> SVDDFISTETPIALNNLLCNVGPDGCRAFGTSAGAVIASPSTIDPDYYYMWTRDSALVFKNLIDRFTETYDAGLQRRIEQYITAQVTLQGLSNPSGSLADGSGLGEPKFELTLKPFTGNWGRPQRDGPALRAIALIGYSKWLINNNYQSTVSNVIWPIVRNDLNYVAQYWNQTGFDLWEEVNGSSFFTVANQHRALVEGATLAATLGQSGSAYSSVAPQVLCFLQRFWVSSGGYVDSNINTNEGRTGKDVNSVLTSIHTFDPNLGCDAGTFQPCSDKALSNLKVVVDSFRSIYG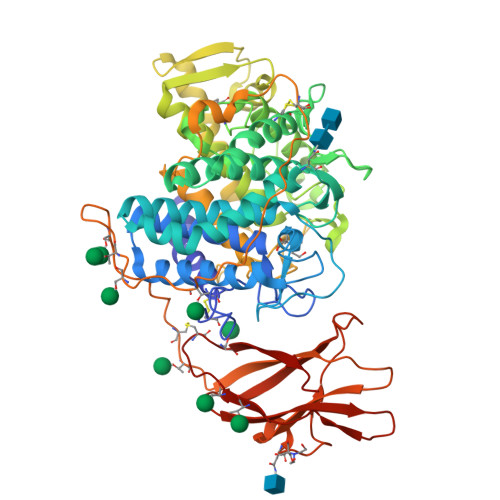VNKGIPAGAAVAIGRYAEDVYYNGNPWYLATFAAAEQLYDAIYVWKKTGSITVTATSLAFFQELVPGVTAGTYSSSSSTFTNIINAVSTYADGFLSEAAKYVPADGSLAEQFDRNSGTPLSALHLTWSYASFLTATARRAGIVPPSWANSSASTIPSTCSGASVVGSYSRPTATSFPPSQTPKPGVPSGTPYTPLPCATPTSVAVTFHELVSTQFGQTVKVAGNAAALGNWSTSAAVALDAVNYADNHPLWIGTVNLEAGDVVEYKYINVGQDGSVTWESDPNHTYTVPAVACVTQVVKEDTWQS> MGASMTGGQQMGAPITAYAQQTRGLLGCIITSLTGRDKNQVEGEVQIVSTATQTFLATCINGVCWTVYHGAGTRTIASPKGPVIQMYTNVDQDLVGWPAPQGSRSLTPCTCGSSDLYLVTRHADVIPV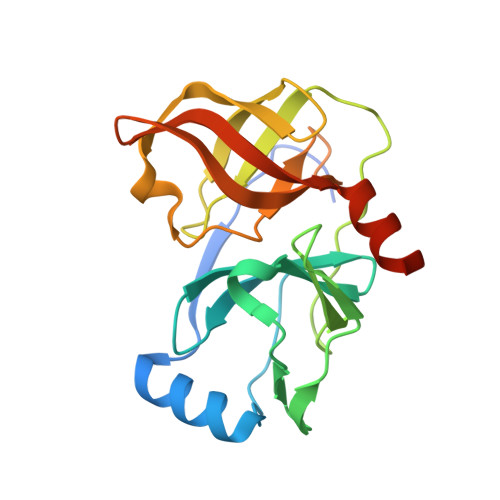RRRGDSRGSLLSPRPISYLKGSSGGPLLCPAGHAVGLFRAAVCTRGVAKAVDFIPVENLETTMRSGSHHHHHH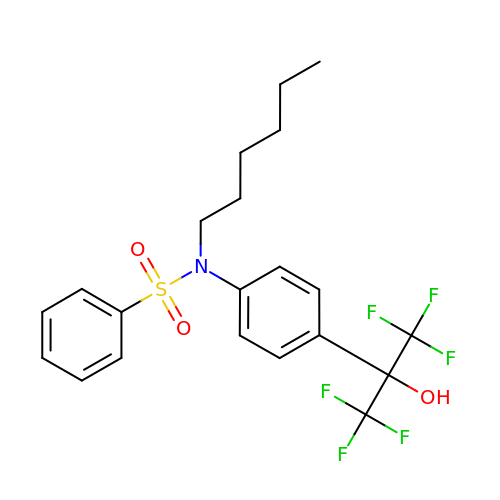N-[4-(1,1,1,3,3,3-hexafluoro-2-hydroxypropan-2-yl)phenyl]-N-hexylbenzenesulfonamide | C21 H23 F6 N O3 S | SASBEAQTFLSSHQ-UHFFFAOYSA-N>[10x]GSHMAHQPSDTIAGLYEAFNSGDLETLRELIAPDAVIHLPGTAGDAEHPPGTPRDREGWLGVWQFTQAFFPDMTATVQD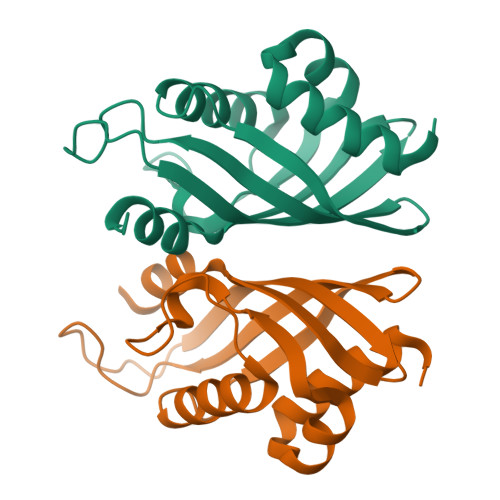IVQTGDLVATRCVARGTHSIEFMGVPPTGRPFEMTMLNMSRVRDGRIVEHWTISDNVTMLAQLGVKASL>[2x]MATIEEIKEVVLKPYTNHRQLTIREVETISINLIDLLITKDVKDARTMKYISRFLTKQDYADLVQERNLVKR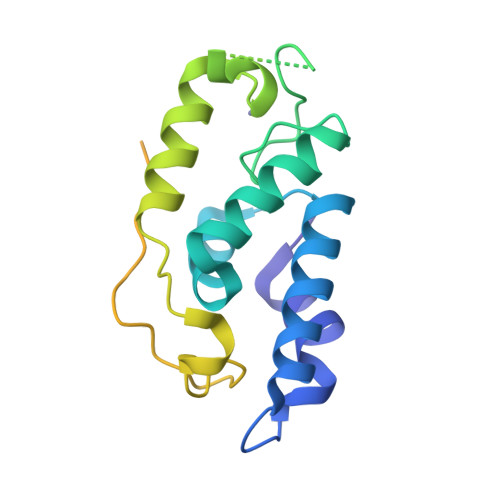CGYPLCSKSQARVRDPFADVQMTNFLRQNNPYAYLTEYCTKAHFRCSQFYQFQLSDEALFARVGVHLDDYEPPSEIQLLEEVLARESDVKQMIRGMTDLKLADDDSREEMERDISDMLADIKIVEINEPNIIGDLGRDRLEHHHHHH> ASLTEIEHLVQSVCKSYRETCQLRLEDLLRQRSNIFSRE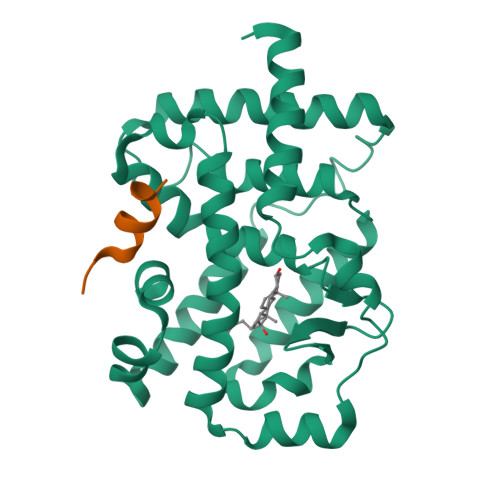EVTGYQRKSMWEMWERCAHHLTEAIQYVVEFAKRLSGFMELCQNDQIVLLKAGAMEVVLVRMCRAYNADNRTVFFEGKYGGMELFRALGCSELISSIFDFSHSLSALHFSEDEIALYTALVLINAHRPGLQEKRKVEQLQYNLELAFHHHLCKTHRQSILAKLPPKGKLRSLCSQHVERLQIFQHLHPIVVQAAFPPLYKELFS;> KHKILHRLLQDS>GSMADLDDIKDGKDFRTDQPQKNIPFTLKGCGALDWGMQSRLSRIFNPKTGKTVMLAFDHGYFQGPTTGLERIDIN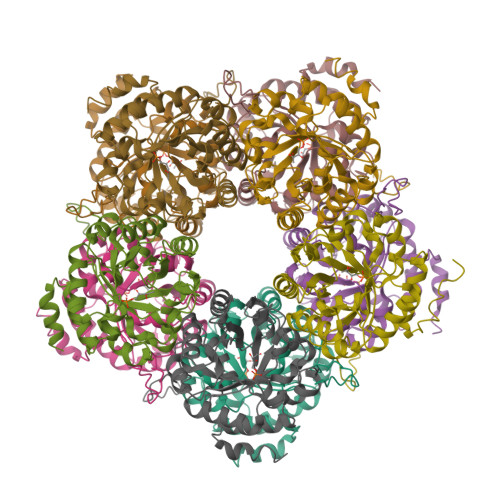IAPLFEHADVLMCTRGILRSVVPPATNRPVVLRASGANSILAELSNEAVALSMDDAVRLNSCAVAAQVYIGSEYEHQSIKNIIQLVDAGMKVGMPTMAVTGVGKDMVRDQRYFSLATRIAAEMGAQIIATYYVEKGFERIVAGCPVPIVIAGGKKLPEREALEMCWQAIDQGASGVDMGRNIFQSDHPVAMMKAVQAVVHHNETADRAYELYLSEKQ[10x]1-phenyl-3-[4-(1H-tetrazol-5-yl)phenyl]urea 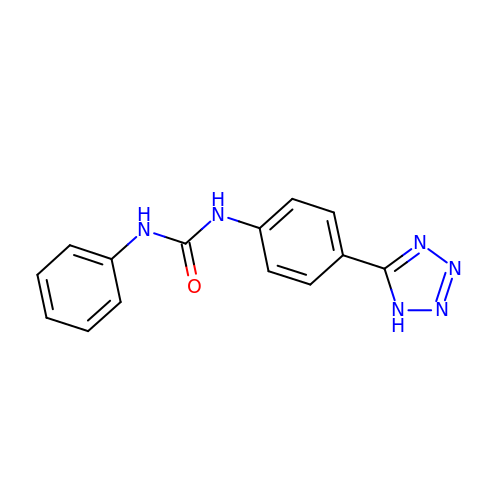| C14 H12 N6 O | KTIWLNFSBOCUHG-UHFFFAOYSA-N> MGSHHHHHHDITSLYKKAGSENLYFQMKLRYLNILKEKLGREPTFVELQAFSVMWSEHCGYSHTKKYIRRLPKTGFEGNAGVVNLDDYYSVAFKIESHNHPSAIEPYNGAATGVGGIIRDVLAMGARPTAIFDSLHMSRIIDGIIEGIADYGNSIGVPTVGGELRISSLYAHNPLVNVLAAGVVRNDMLVDSKASRPGQVIVIFGGATGRDGIHGASFASEDLTGDKATKLSIQVGDPFAEKMLIEAFLEMVEEGLVEGAQDLGAGGVLSATSELVAKGNLGAIVHLDRVPLREPDMEPWEILISESQERMAVVTSPQKASRILEIARKHLLFGDVVAEVIEEPVYRVMYRNDLVMEVPVQLLANAPEEDIVEYTPGKIPEFKRVEFEEVNAREVFEQYDHMVGTDTVVPPGFGAAVMRIKRDGGYSLVTHSRADLALQDTYWGTLIAVLESVRKTLSVGAEPLAITNCVNYGDPDVDPVGLSAMMTALKNACEFSGVPVASGNASLYNTYQGKPIPPTLVVGMLGKVNPQKVAKPKPSKVFAVGWNDFELEREKELWRAIRKLSEEGAF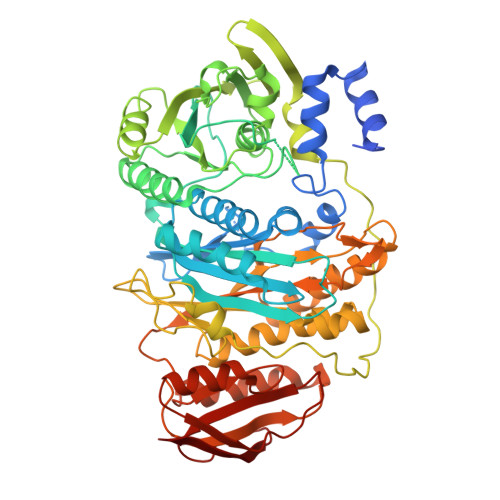ILSSSQLLTRTHVETFREYGLKIEVKLPEVRPAHQMVLVFSERTPVVDVPVKEIGTLSR> GSHMLSDEQMQIINSLVEAHHKTYDDSYSDFVRFRPPVREGPVTRSASRAASLHSLSDASSDSFNHSPESVDTKLNFSNLLMMYQDSGSPDSSEEDQQSRLSMLPHLADLVSYSIQKVIGFAKMIPGFRDLTAEDQIALLKSSAIEIIMLRSNQSFSLEDMSWSCGGPDFKYCINDVTKAGHTLEHLEPLVKFQVGLKKLKLHEEEHVLLMAICLLSPDRPGVQDHVRIEALQDRLCDVLQAYIRIQHPGGRLLYAKMIQKLADLRSLNEEHSKQYRSLSFQPEHSMQLTPLVLEVFGSEVS;> RHKILHRLLQEGSPS

The activities of 1,25D3 are mediated by its binding to the Vitamin D Receptor (VDR, also termed NR1I1), a ligand-dependent transcription factor that belongs to the nuclear receptor superfamily. The 1,25D3 plays a key role in calcium homeostasis by promoting VDR activities in the intestines, bones and kidneys, and is involved in a wide spectrum of biological pathways, including cell differentiation and immune responses. The VDR/RXR heterodimers bind to genomic locations, known as vitamin D response elements (VDRE), within the regulatory regions of their target genes to modulate gene transcription in concert with various co-regulatory molecules. In the present study, by solving the crystal structure of wild type (WT)- and VDRgem-bound to BXL-62, we identify the mechanisms underlying the high potency of the C-20-modified analogs to induce the transcriptional activities of VDR.

In addition, Gemini-72 restores the transcriptional activity of VDRgem (L337H in zebrafish or L309H in humans), a point-mutated VDR unresponsive to 1,25D3. In addition, we show that BXL-62 is able to restore the transcriptional activity of the VDRgem variant, that was designed to respond selectively to gemini ligands and to be unresponsive to 1,25D3. To determine whether similar structural modifications are observed in the VDR variants, BXL-62 in complex with zVDRgem (L337H) was crystallized, solved, and refined to 2.4 Å. All of the interactions observed in the zVDR WT-BXL-62 complex were conserved in zVDRgem-BXL-62, notably the specific and tighter interactions involving the C-20 cyclopropyl moiety. The BXL-62 interacted more strongly with H337 of zVDRgem through the C-21 atom of the cyclopropyl than that of zVDR WT. The stronger interactions formed by the side chain of BXL-62 with residues of H6, H7, and of the C-terminus stabilized the active conformation of VDRgem, in contrast to the 1,25D3 that exhibited weakened hydrogen bonds between 25-OH and zHis333 and zHis423. In contrast, 1,25D3 failed to stabilize the interaction with the zVDRgem His423. This different interaction between BXL-62 and 1,25D3 with His423 is due to the His337 having a stronger contact probability with His423 in the zVDRgem-BXL-62 complex. The presence of the cyclopropyl moiety prevented the interaction between these two histidine residues, while showing an increased interaction with His423. Taken together, these results demonstrate that the addition of the cyclopropyl to the 1,25D3 skeleton is sufficient to restore the VDRgem agonist conformation and dynamics.> SMSSPLLESSFEPSEPAPQQALYRTAGNPAPRTLLDVLDATAAAHPQAIALDTGSEALTYRDLCIEIERRARQLRDRGIGPGDRVGVRVPSGTAELYLSILAVLRSGAAYVPVDADDPDERAATVFREAAVCAVLGPDGPLPGPARPLGDPRSAGPQDDAWIIFTSGSTGAPKGVAVSHRSAAAFVDAEADLFCQDQPLGPGDRVLAGLSVAFDASCEEMWLAWRYGACLVPAPRALVRAGHELGPWLVERGITVVSTVPTLAALWPDEAMRRVRLLIVGGESCPAGLVDRFAGPGREMWNTYGPTETTVVACAARLLPGEPVRIGLPLKGWQLAVVDRTGQPVPFGAEGELLISGVGTARYLDPAKDAERFRPDDALGAARVYRTGDLVRAEPEGLLFVGRADDQIKLGGRRIELGEIDAALAA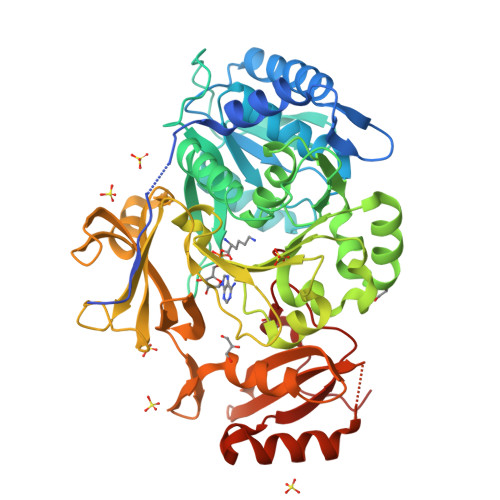LPGVRGAAAAVQTTPAGTQVLVGYVVPEQRTADGSSFQQDKARALLQERLPAQLVPVLAEVESLPTRTSGKVDRKALPWPLPSA(5-methyl-1,2-oxazol-3-yl)methanamine | C5 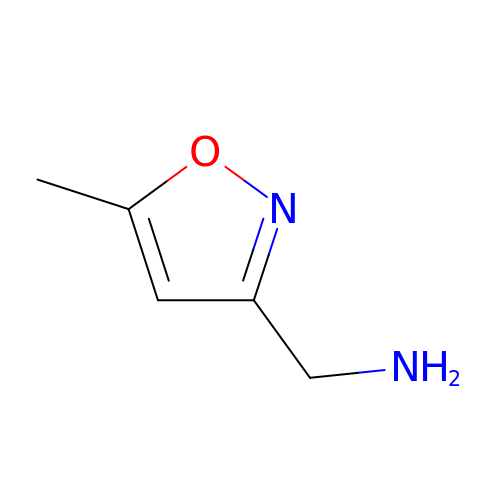H8 N2 O | AZVWIMLQRLKLHH-UHFFFAOYSA-N> MGSDKIHHHHHHENLYFQGHMIKYYNINGQQVPVENATLHVSDLSILRGYGIFDYFLAREGHPLFLDDYLNRFYRSAAELYLEIPFDKAELRRQIYALLQ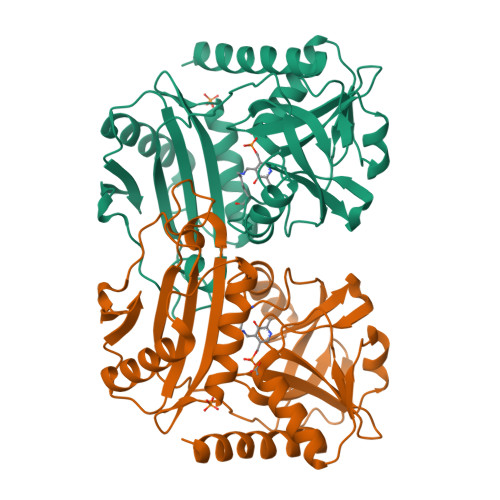ANEVREAGIRLVLTGGYSPDGYTPVNPNLLIMMYDLPASAWEFSAQGIKIITHPFQRELPEVKTINYSTGIRMLKTIKERGATDLIYVDQGEWIRESARSNFFLVMPDNTIVTADEKILWGITRRQVIDAAREAGYAVEERRIHITELDQAREAFFTSTIKGVMAIGQIDDRVFGDGTIGKVTQELQDLFVGKVKAYLETC>GSHMASMNAPISAEEQMIRAFVKSVEYMSPRKIGALVAIQRVRTLQEYISTGIPLDAKISAELLINIFIPNTPLHDGAVIIKEERIAVTSAYLPLTKNTGISKEFGTRHRAAIGLSEV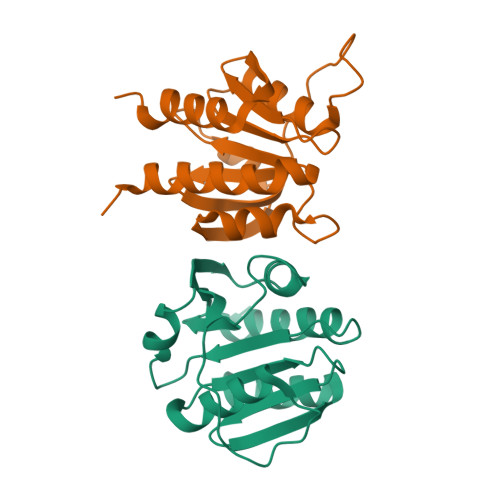SDALTFVVSEETGGISITYNGRFKHNLTLDEFETELREILLPKEEVGLSFKERLLGGWKHEKK[6x]> MASMTGGQQMGRGSEFMTAAGAAQAPIVAGHPLLGSMNDLLNDPLATYLRARRDHGDVVRFRAGPPGLRADIYAVFSAEGAQQVLATESGNFRKDNVFYGELRDSVGNGLLTSQDATYLRQRRLVQPLFTRRRVDGYAGQVADEAAGLAEAWRGIPGGGVELVGEMHRFALRVVGRILFGTDMETTFEVIERTLPLLQEYALKRGLAPVRTPRTWPTPANRRAARTQAELFALCDGIIDSRRNRKNEGDGGEESGEDLVTLLVRAGNAEDGSLDAAELREQVLIFLLAGHETTATALAFALHLLARHPEQQRRVRDEADRVLGGPGGRAPTAADMEALPYLTMVLKEAMRLYPSAPVIGRRAVADAEVDGVRIPAGADLFVSPWVTHRHPDYWPDPERFDPE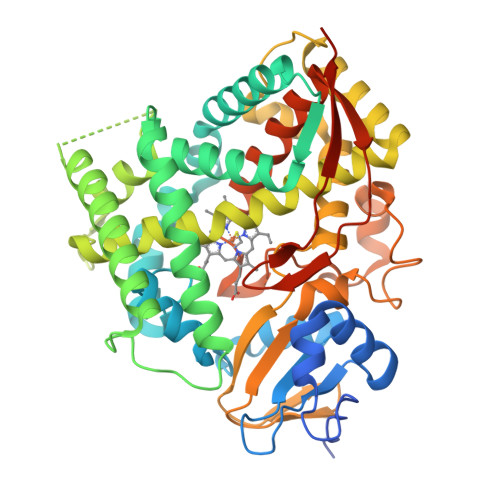RFTPEAEAGRPRYAWFPFGGGPRACIGQHLSMLESVLGLAVLIREFEFEAVGEEEVPLGAGITLLAKGPARCRVIPRSSGPRSSHHHHHH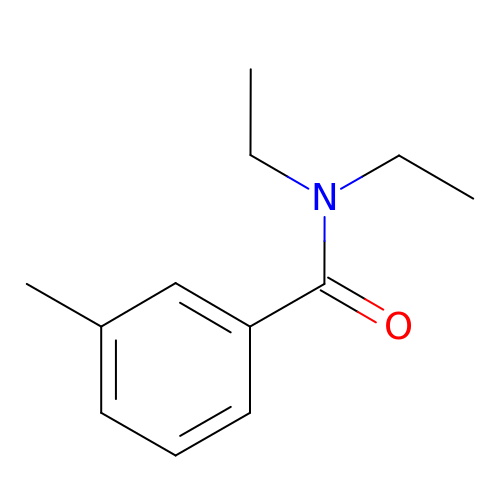N,N-diethyl-3-methylbenzamide | C12 H17 N O | MMOXZBCLCQITDF-UHFFFAOYSA-N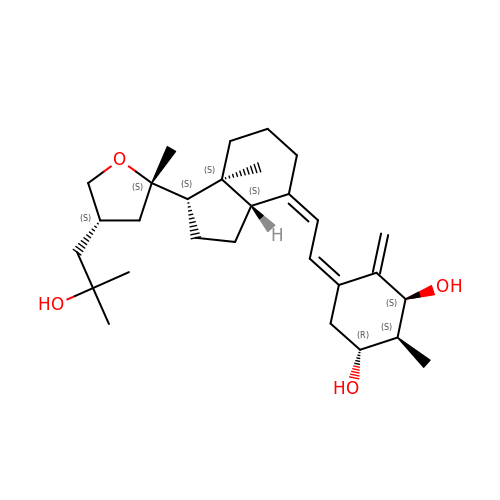(1S,2S,3R,5Z,7E,14beta,17alpha)-17-[(2S,4S)-4-(2-hydroxy-2-methylpropyl)-2-methyltetrahydrofuran-2-yl]-2-methyl-9,10-secoandrosta-5,7,10-triene-1,3-diol | C29 H46 O4 | CDTXSCLKUNDXBZ-SIYPKADPSA-N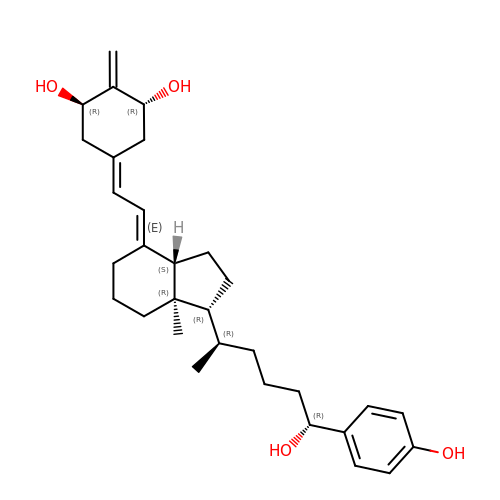(1~{R},3~{R})-5-[(2~{E})-2-[(1~{R},3~{a}~{S},7~{a}~{R})-1-[(2~{R},6~{R})-6-(4-hydroxyphenyl)-6-oxidanyl-hexan-2-yl]-7~{a}-methyl-2,3,3~{a},5,6,7-hexahydro-1~{H}-inden-4-ylidene]ethylidene]-2-methylidene-cyclohexane-1,3-diol | C31 H44 O4 | YBYKLULOUNBMJL-PJZOPEKWSA-N> MHEWALADAIVRTVLDYAQREGASRVKAVRVVLGELQDVAEDIVKFAMEQLFAGTIAEGAEIEFVEEEAVFK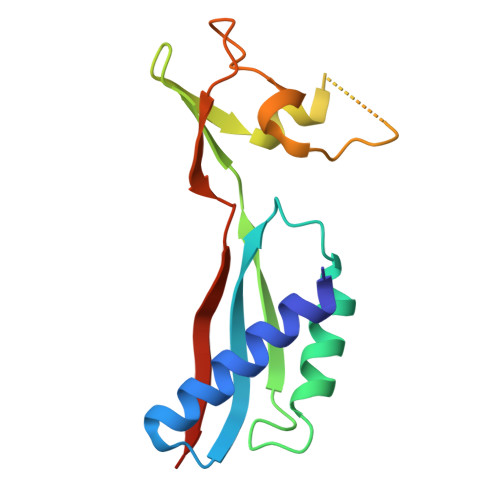CRNCNYEWKLKEVKDKFDERIKEDIHFIPEVVHAFLACPKCGSHDFEVVKGRGVYVAGIKIEKEGGS MbtI from Mycobacterium tuberculosis (Mtb) is a Mg2+-dependent salicylate synthase, belonging to the chorismate-utilizing enzyme (CUE) family. MbtI converts chorismate to salicylate via a two-step mechanism, with the release of pyruvate. As a fundamental player in iron acquisition, MbtI promotes the survival and pathogenicity of Mtb in the infected host. MbtI is known to exist in two possible conformations, generally referred to as “open” and “closed”, depending on the position of two flexible loops relative to the active site, as extensively analyzed in our previous work.

Moreover, we describe a new crystal structure of MbtI in open conformation and in complex with the known inhibitor methyl-AMT, suggesting that in vitro potency is not related to the observed enzyme conformation. Interestingly, in our MbtI-methyl-AMT model, all protomers were rather found to be in an open state, with poor or no supporting electron density for most of the mobile loops (residues 273–284 and 327–331) in three out of the four protomers in the ASU. However, these regions could be traced entirely in the fourth protomer (chain B), mostly due to stabilizing packing interactions involving the Gly277-Ile280 β-turn. However, contrarily to the previous complex, and despite an equivalent pose in the active site, no hydrogen bond interaction could be observed in our complex between the methyl-AMT enolpyruvyl side chain and the hydroxyl group of Thr271, supporting the hypothesis of a correlation between this interaction and the closed state of the enzyme. These findings are in line with our conclusion that the overall MbtI conformation, and most notably the closure of the active site lid, does not correlate with the inhibitor potency in vitro, with different protomers showing different conformations in the presence of the same compound. We also described a novel, higher-resolution complex of MbtI with the known inhibitor methyl-AMT, in which the enzyme, conversely, adopted an open conformation.

>[4x]HMSELSVATGAVSTASSSIPMPAGVNPADLAAELAAVVTESVDEDYLLYECDGQWVLAAGVQAMVELDSDELRVIRDGVTRRQQWSGRPGAALGEAVDRLLLETDQAFGWVAFEFGVHRYGLQQRLAPHTPLARVFSPRTRIMVSEKEIRLFDAGIRHREAIDRLLATGVREVPQSRSVDVSDDPSGFRRRVAVAVDEIAAGRYHKVILSRCVEVPFAIDFPLTYRLGRRHNTPVRSFLLQLGGIRALGYSPELVTAVRADGVVITEPLAGTRALGRGPAIDRLARDDLESNSKEIVEHAISVRSSLEEITDIAEPGSAAVIDFMTVRERGSVQHLGSTIRARLDPSSDRMAALEALFPAVTASGIPKAAGVEAIFRLDECPRGLYSGAVVMLSADGGLDAALTLRAAYQVGGRTWLRAGAGIIEESEPEREFEETCEKLSTLTPYLVARQ> SNAMKPENKIPVLTRLSDEMTAVV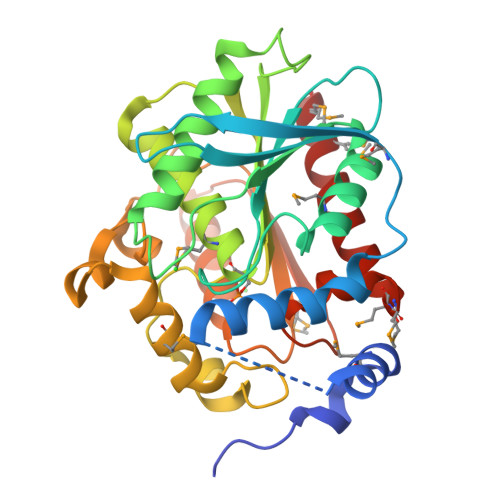NFQQPGLPPWPADGDIETQRQYYLLERRFWNADAPSMTTRTCAVPTPYGDVTTRLYSPQPTSQATLYYLHGGGFILGNLDTHDRIMRLLARYTGCTVIGIDYSLSPQARYPQAIEETVAVCSYFSQHADEYSLNVEKIGFAGDSAGAMLALASALWLRDKHIRCGNVIAILLWYGLYGLQDSVSRRLFGGAWDGLTREDLDMYEKAYLRNDEDRESPWYCLFNNDLTRDVPPCFIASAEFDPLIDDSRLLHQTLQAHQQPCEYKMYPGTLHAFLHYSRMMTIADDALQDGARFFMARMKTPR We describe here the use of an artificial cofactor employing the well‐known biotin‐streptavidin system to catalyze a Baylis‐Hillman reaction. As protein host, we chose streptavidin, as it can be easily crystallized and thereby supports the design process. There are several examples using streptavidin as the host for these cofactors, since its natural ligand biotin binds strongly (K d∼10−15 M) and is easy to modify with catalysts at the carboxylic acid group. No enzyme is known to naturally catalyze the Baylis‐Hillman reaction, a very versatile and atom‐economic C−C bond forming reaction for the production of various functionalized compounds and intermediates of active pharmaceutical ingredients (APIs).

We chose a derivative of DMAP as the artificial cofactor due to its low steric demand, which will facilitate its inclusion into the protein scaffold. The protein host around the cofactor was rationally designed on the basis of high‐resolution crystal structures obtained after each variation of the amino acid sequence. The location of the catalyst is in a shallow cavity at the surface of the protein. The system was evolved through repeated cycles of mutagenesis, activity tests, and structure determination. According to the presented structures and calculations the catalytically active site is too shallow to undergo interactions with 1.

>MASMTGGQQMGRDEAGITGTWYNQLGSTFIVTAGADGALTGTYESAAGKAESRYVLTGRYDSAPATDGSGTALGWTVAWKNNYRNAHSATTWSGQYVGGAEARINTQWLLTAGATEANGWASTYVGHDTFTKVKPSAASIDAAKKAGVNNGNPLDAVQQ[2x]>MAKLETVTLGNIGKDGKQTLVLNPRGVNPTNGVASLSQAGAVPALEKRVTVSVSQPSRNRKNYKVQVKIQNPTACTANGSCDPSVTRQAYADVTFSFTQYSTDEERAFVRTELAALLASPLLIDAIDQLNPAY[3x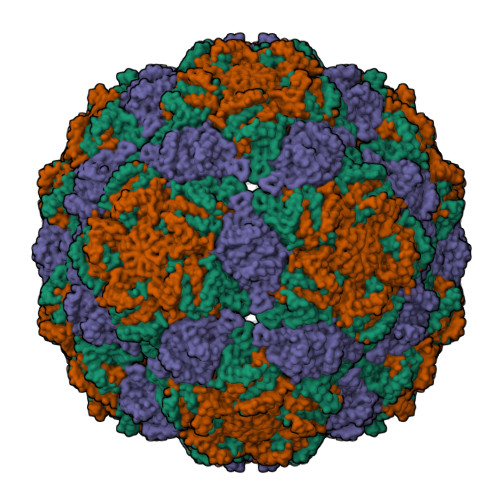]>[3x]XQARSDIEKLKEAIRDTNKAVQSV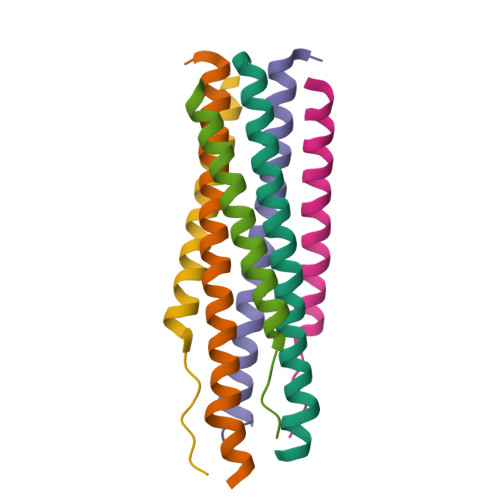QSSIGNLIVAIKSVQDYVNKEIVPSIARX;>XVALDPIDXSIVLNKIKSQLEESKEWIRRSNKILDSIX[3x]> MSLIERGLAKLTINAYKDREGKIRAGTLQAMYNPDSLQLDYQTDYQQSQAINSEKQSSIYVQAKPAGLSLELIFDATMPGNKTPIEEQLMQLKQLCSVDATSNETRFLQVKWGKMRWESRGYFAGRAKSLSVNYTLFDRDATPLRVRVILALVADESLVLQETEQNLQSPAKIA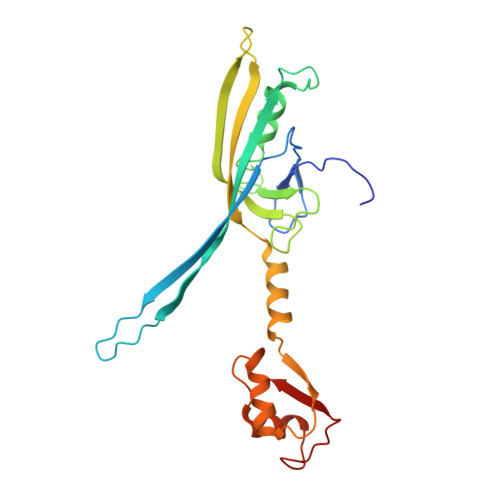LRIQDGVSLALMAASTASTLSGGVDYLTLAWQNGLDNLNGFVPGEILQATRGDES> MAKREPIHDNSIRTEWEAKIAKLTSVDQATKFIQDFRLAYTSPFRKSYDIDVDYQYIERKIEEKLSVLKTEKLPVADLITKATTGEDAAAVEATWIAKIKAAKSKYEAERIHIEFRQLYKPPVLPVNVFLRT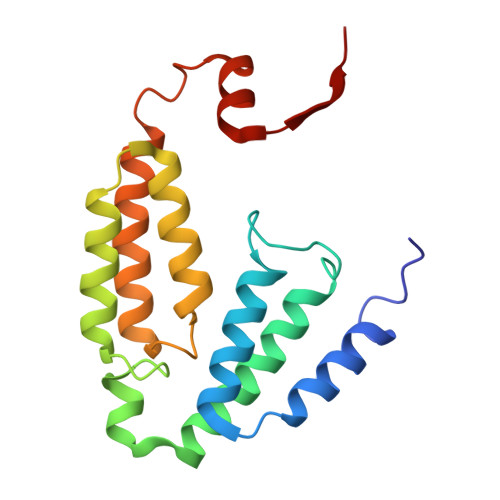DAALGTVLMEIRNTDYYGTPLEGLRKERGVKVLHLQA> DHNTEEMENSADRVTTQTAGNTAINTQSSLGVLCAYVEDPTKSDPPSSSTDQPTTTFTAIDRWYTGRLNSWTKAVKTFSFQAVPLPGAFLSRQGGLNGGAFTATLHRHFLMKCGWQVQVQCNLTQFHQGALLVAMVPETTLDVKPDGKAKSLQELNEEQWVE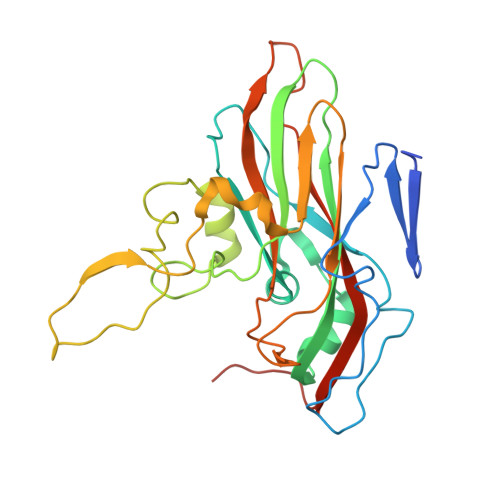MSDDYRTGKNMPFQSLGTYYRPPNWTWGPNFINPYQVTVFPHQILNARTSTSVDVNVPYIGETPTQSSETQNSWTLLVMVLVPLDYKEGATTDPEITFSVRPTSPYFNGLRNRYTAGTDEEQ S100 proteins are a subfamily of EF-hand calcium-binding proteins found primarily in vertebrate animals. S100 proteins are comprised of two EF-hand helix-loop-helix Ca2+-binding motifs. They are distinguished from other EF-hand proteins by a unique, noncanonical S100-specific Ca2+ binding loop in the N-terminal EF-hand, an intrinsic dimeric architecture, and the binding of Zn2+ and other transition metals at the dimer interface. S100A7 functions in the protection of the skin and mucous membranes and is a biomarker in inflammatory skin disease. The binding of Zn2+ has been shown to be a central factor in the antimicrobial activity of S100A7; sequestration of Zn2+ by S100A7 starves invading pathogens of this essential metal, a mechanism termed nutritional immunity.

Based on this observation and careful analysis of secondary structure predictions, a construct truncating the protein at His100 (mouse S100A7 tailless [mS100A7ΔC]) was prepared and used for subsequent crystallization trials. Crystallization trials performed on mS100A7ΔC yielded diffracting crystals in the presence of Ca2+, and the structure could be refined to 1.69 Å resolution. The crystal was orthorhombic, in space group P212121, and contained one homodimer per asymmetric unit. The structure of mS100A7 revealed the canonical S100 protein dimeric architecture; each protomer is organized into two EF-hands with the hydrophobic core integrated across the dimer interface. Like all Ca2+-loaded full-length S100 proteins, mS100A7 occupies an open conformation with HIII shifted out from the core exposing a hydrophobic cleft. The Ca2+ ion is coordinated in a canonical pentagonal bipyramidal geometry by the backbone carbonyl oxygen atoms of Ala21, Glu24, Asp26, and Thr29, plus the critical, highly conserved bidentate carboxylate of Glu34 and a structural water molecule stabilized by an H-bond to Thr29 Oγ1. The Ca2+ ion is coordinated by side chain oxygen atoms of Asp66, Asn68, and Asp70, plus the backbone carbonyl oxygen of Gln72, the critical, highly conserved bidentate Glu77, and a water molecule stabilized by a bifurcated H-bond with Asp70 Oδ and Cys74 SH. The two symmetrically disposed canonical Zn2+ binding sites at the dimer interface, composed of the side chains of His18 and Glu28 from one chain and His 90 and His94 from the other, are all visible in the structure. Nevertheless, the overall geometry of these sites is set up for tetrahedral coordination, and in fact, a Na+ ion is found in both sites. The most significant difference between the two protein structures is due to mS100A7 having a standard N-terminal S100-specific Ca2+-binding loop (Ala21-Glu34), whereas this loop in hS100A7 is truncated to 12 residues (Tyr19-Ser30).

>[2x]MPDTPVEDSLFQIIHCFHHYAAREGDKETLSLEELKALLLDSVPRFMDTLGRRQPYYITELFRAADKNKDNQICFDEFLYILGKLVKDYHLQFHRQLCAH>MAHHHHHHVGTMENENKPNVANFEAAVAAKDYEKACSELLLILSQLDSNFGGIQEIEFEYPAQLQDLEQEKIVYFCTRMATAITTLFSDPVLEISDLGVQRFLVYQRWLALIFASSPFVNADHILQTYNREPNRKNSLEIHLDSSKSSLIKFCILYLPESNVNLNLDVMWNISPELCASLCFALQSPRFIGTSTAFNKRATILQWFPRHLDQLKNLNNIPSAISHDVYMHCSYDTSVNKHDVKRALNHVIRRHIESEYGWKDRDVAHIGYRNNKPVMVVLLEHFHSAHSIYRTHSTSMIAAREHFYLIGLGSPSVDQAGQEVFDEFHLVAGDNMKQKLEFIRSVCESNGAAIFYMPSIGMDMTTIFASNTRLAPIQAIALGHPATTHSDFIEYVIVEDDYVGSEECFSETLLRLPKDALPYVPSALAPEKVDYLLRENPEVVNIGIASTTMKLNPYFLEALKAIRDRAKVKVHFHFALGQSNGITHPYVERFIKSYLGDSATAHPHSPYHQYLRILHNCDMMVNPFPFGNTNGIIDMVTLGLVGVCKTGAEVHEHIDEGLFKRLGLPEWLIANTVDEYVERAVRLA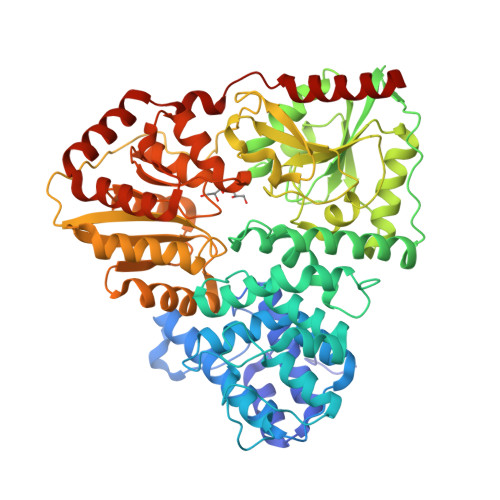ENHQERLELRRYIIENNGLNTLFTGDPRPMGQVFLEKLNAFLKEN[2x]>[3x]LQQPLLVATRVIPPFVLSNKGELSGFSIDLWRSIATQIGIESKLIEYSSVPELISAIKDNKVNLGIAAISITAEREQNFDFSLPIFASGLQIMVRNLESGTGDIRSIDDLPGKV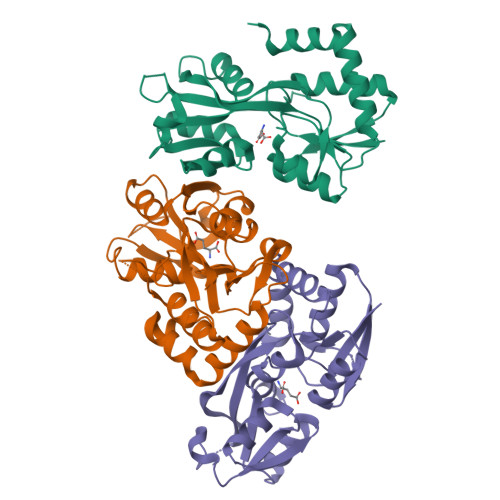VATTAGSTAATYLREHHISVLEVPKIEEAYKALQTKKADAVVFDAPVLLFYAANEGKGKVEIVGSILREESYGIILPNNSPYRKPINQALLNLKENGTYQSLYDKWFDPKNSLE> IEMKPHPWFFGKIPRAKAEEMLSKQRHDGAFLI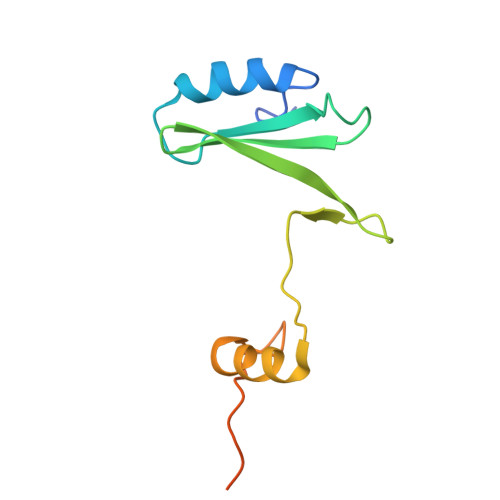RESESAPGDFSLSVKFGNDVQHFKVLRDGAGKYFLWVVKFNSLNELVDYHRSTSVSRNQQIFLRDIEQVPQQPTYVQHHHHHH2-fluoro-ATP | C10 H15 F N5 O13 P3 | 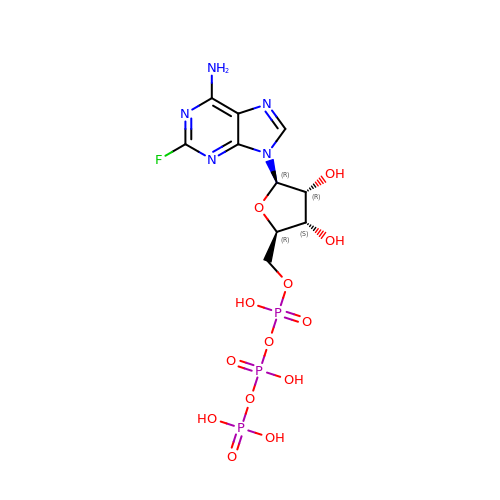PIOKUWLZUXUBCO-UUOKFMHZSA-N> 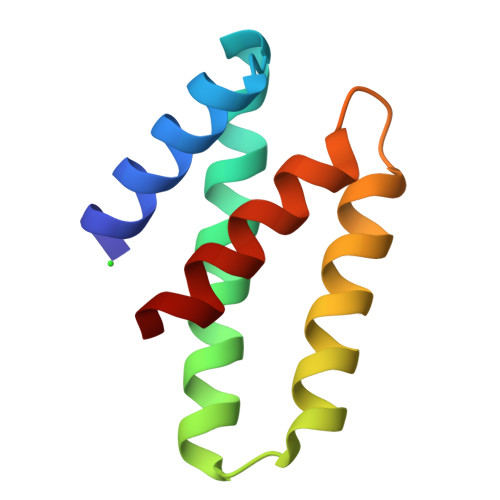YHKLRLAIKEICKTDGIPNIKWGMYIAFGEKLLKSYLKMKAGSASSDMIAEYINNAISAFSSRTGISQETAQKIADFITSNY>MAHHHHHHMNGFDRELKNRVLGMVPQATVSSTQILTDWPELVKRVENHPHVTGVAPFTQLQGMLTAQGQVAGIMVTGIDPKYEKNVSIIQNHIVAGSLDSLKKGEFGIVLGKDMADSLGLRLNDSVTLVLPEATPSPAGVVPRFKRFKVVGIFSVGAEVDSMVGYIALYDASTLLRLPDGAQGVRLKLDDIFAAPQVADDIVKNLPSNFYATNWTYTHGNLFNAIQMEKT[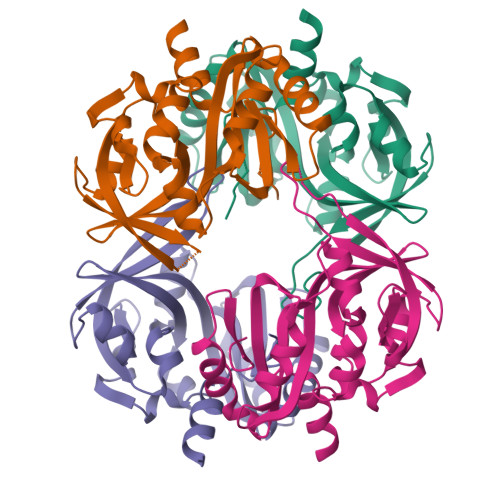4x]>[4x]MGSSHHHHHHSQDPNSSSMSNNTISTKPALHFLDINATEVKKYPTAIQDIIINRSFDGMIIRGVFPRDTMEQVARCLEEGNDGGMKSILNKNEEFGTKVAQIYGHAIVGQSPDLKDYFASSAIFRQACRTMFQGSPDFEEQVESIF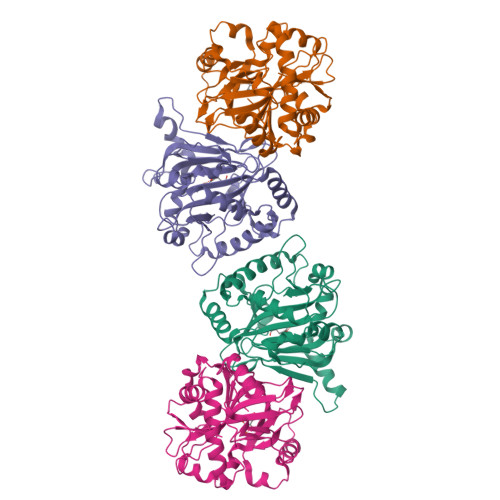HSLSELPVEIPTGPEGQTYTPATIRLLLEGREIAVHVGNDFLLMPAANHLKTLLDLSDQLSYFIPLTVPEAGGELVVYSLEWNPQEASKYAQMQEYMDDVESKIKSNQSQSVAYAPGPGDMLLFNGGRYYHRVSEVIGNSPRRTIGGFLAFSKQRNKIYYWS Among the most interesting of the discovered proteins was CotE, an 81 kDa protein comprising an N-terminal domain homologous to 1-Cys peroxiredoxins, a central cysteine-rich interdomain region and a C-terminal domain with homology to family 18 glycosyl hydrolases (GH18). CotE is a bifunctional spore-coat protein with peroxiredoxin and chitinase domains that are implicated in colonization. Insertional mutagenesis showed that cotE is not essential for spore integrity; however, in animal models of CDI, when CotE is absent the capacity of spores to colonize the intestine and induce virulence is markedly reduced.

To obtain unliganded CotE(349–712), the first Ni–NTA column-chromatography purification procedure was modified so that after the binding and washing steps, the column was washed with buffer C (buffer A containing 2 M guanidine hydrochloride) to partially unfold the immobilized protein and allow the dissociation of endogenous ligand(s). The partially unfolded/refolded protein was crystallized in a different crystal form (P6122). Solution of the structure and refinement against data extending to ∼2.1 Å resolution revealed that the substrate-binding groove was indeed empty. However, the structure proved to be of a 3D domain-swapped dimer. In this structure, domain exchange takes place at residue Lys627. Thus, 244 Cα atoms in the residue range 368–623 can be superposed with an r.m.s.d. of 0.44 Å, while similarly 78 Cα atoms of residues 627–708 can be superposed with an r.m.s.d. of 0.43 Å. In almost all instances 3D domain swapping is a crystallographic artefact and there is no evidence that the 3D domain-swapped dimer of CotE(349–712) is physiologically significant. It is nevertheless structurally interesting since it involves (i) the exchange of a strand, β8, from the β-barrel and (ii) the breakage of the intramolecular disulfide bond between Cys376 and Cys670 and the formation of an intermolecular equivalent. The 3D domain-swapped CotE(349–712) structure reported here is therefore the second example, with the distinction that it is the C-terminal strand 8 of the barrel that is swapped.

> GPAMKTLKDSKKLVRPQITDPYNPIVENANCPDINPIVAEYVLGNPTNVDAQLLDAVIFAFAEIDQSGNLFIPYPRFLNQLLALKGEKPSLKVIVAIGGWGAEGFSDAALTPTSRYNFARQVNQMINEYALDGIDIDWEYPGSSASGITSRPQDRENFTLLLTAIRDVIGDDKWLSVAGTGDRGYINSSAEIDKIAPIIDYFNLMSYDFTAGETGPNGRKHQANLFDSDLSLPGYSVDAMVRNLENAGMPSEKILLGIPFYGRLGATITRTYDELRRDYINKNGYEYRFDNTAQVPYLVKDGDFAMSYDDALSIFLKTQYVLRNCLGGVFSWTSTYDQANILARTMSIGINDPEVLKEELEGIYGQF> MKTLVHVASVEKGRSYEDFQKVYNAIALKLREDDEYDNYIGYGPVLVRLAWHISGTWDKHDNTGGSYGGTYRFKKEFNDPSNA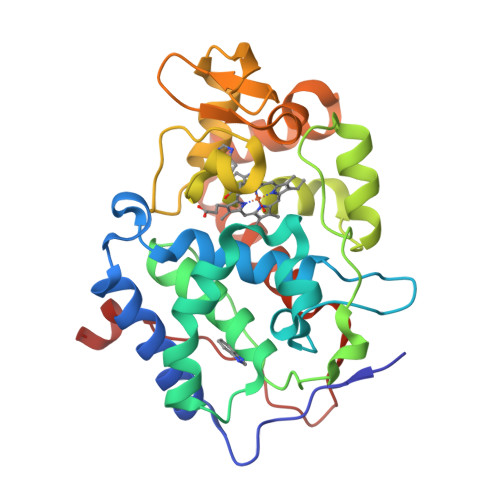GLQNGFKFLEPIHKEFPWISSGDLFSLGGVTAVQEMQGPKIPWRCGRVDTPEDTTPDNGRLPDADKDAGYVRTFFQRLNMNDREVVALMGAHALGKTHLKNSGYEGGGANNVFTNEFYLNLLNEDWKLEKNDANNEQWDSKSGYMMLPTDYSLIQDPKYLSIVKEYANDQDKFFKDFSKAFEKLLENGITFPKDAPSPFIFKTLEEQGL>MLNQELELSLNMAFARAREHRHEFMTVEHLLLALLSNPSAREALEACSVDL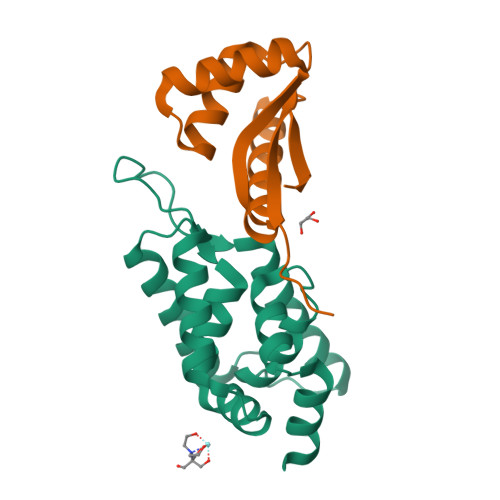VALRQELEAFIEQTTPVLPASEEERDTQPTLSFQRVLQRAVFHVQSSGRNEVTGANVLVAIFSEQESQAAYLLRKHEVSRLDVVNFISHGT[2x];>MGKTNDWLDFDQLAEEKVRDALKPPSMYKVILVNDDYTPMEFVIDVLQKFFSYDVERATQLMLAVHYQGKAICGVFTAEVAETKVAMVNKYARENEHPLLCTLEKA[2x]>[4x]MSADVAGAVIDGAGLGFDVLKTVLEALGNVKRKIAVGIDNESGKTWTAMNTYFRSGTSDIVLPHKVAHGKALLYNGQKNRGPVATGVVGVIAYSMSDGNTLAVLFSVPYDYNWYSNWWNVRVYKGQKRADQRMYEELYYHRSPFRGDNGWHSRGLGYGLKSRGFMNSSGHAILEIHVTKA

Fragaceatoxin C (FraC)11 is a potent haemolysin of the family of actinoporins, defined as a group of ~20 kDa protein toxins produced by sea anemones. Actinoporins are classified as α-helical PFT (α-PFT) because the transmembrane pore is predicted to form an α-helical barrel. The lytic activity of actinoporins on biological membranes is enhanced by the lipid sphingomyelin (SM) and by lipid-phase coexistence. Here we reveal structures of FraC corresponding to four different stages of its activation route, namely the water-soluble form, the lipid-bound form, an assembly intermediate and the transmembrane pore.

In the monomeric form of FraC, the side chain of Phe16 is inserted in a hydrophobic cavity of the β-core region.>SGLDMNISQ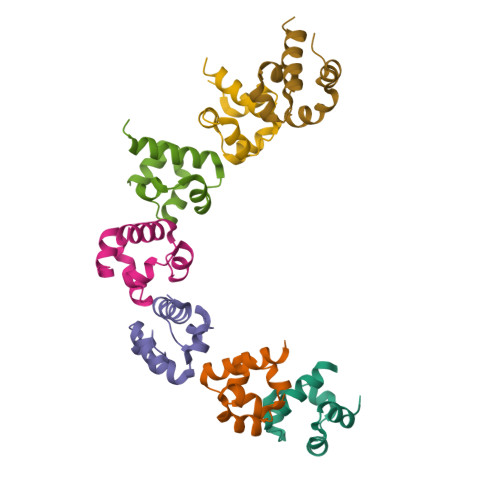FLKSLGLEHLRDIFETEQITLDVLADMGHEELKEIGINAYGHRHKLIKGVERLLGGQQ[7x]>GMSENSSVRHGLTSAQHEVWLAQQLDPRGAHYRTGSCLEIDGPLDHAVLSRALRLTVAGTETLCSRFLTDEEGRPYRAYCPPAPEGSAAVEDPDGVPYTPVLLRHIDLSGHEDPEGEAQRWMDRDRATPLPLDRPGLSSHALFTLGGGRHLYYLGVHHIVIDGTSMALFYERLAEVYRALRDGRAVPAAAFGDTDRMVAGEEAYRASARYERDRAYWTGLFTDRPEPVSLTGRGGGRALAPTVRSLGLPPERTEVLGRAAEATGAHWARVVIAGVAAFLHRTTGARDVVVSVPVTGRYGANARITPGMVSNRLPLRLAVRPGESFARVVETVSEAMSG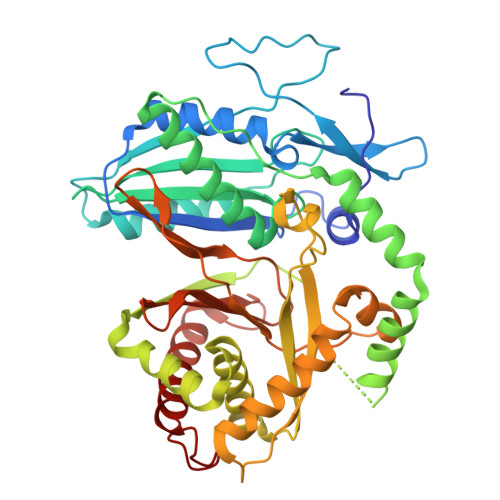LLAHSRFRGEDLDRELGGAGVSGPTVNVMPYIRPVDFGGPVGLMRSISSGPTTDLNIVLTGTPESGLRVDFEGNPQVYGGQDLTVLQERFVRFLAELAADPAATVDEVALLT[2x]> GAMAVLDPEVAQLLSQANEAFVRNDLQVAERLFNEVIKKDARNFAAYETLGDIYQLQGRLNDCCNSWFLAAHLNASDWEFWKIVAILSADLDHVRQAIYCFSRVISLNPMEWESIYRRSMLYKKTGQLARALDGFQRLYMYNPYDANILRELAILYVDYDRIEDSIELYMKVFNANVERREAILAALENALDSSDEESAAEGEDADEKEPLEQDEDRQMFPDINWKKIDAKYKCIPFDWSSLNILAELFLKLAVSEVDGIKTIKKCARWIQRRESQTFW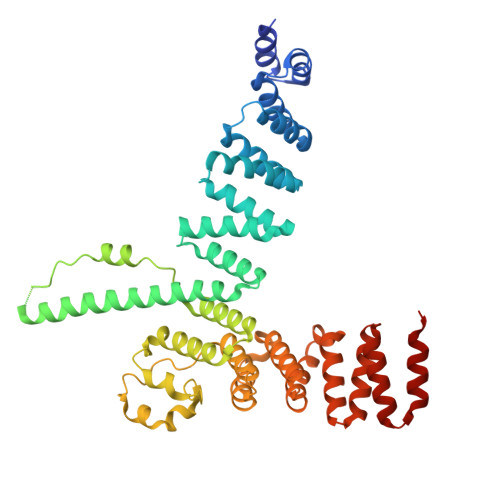DHVPDDSEFDNRRFKNSTFDSLLAAEKEKSYNIPIDIRVRLGLLRLNTDNLVEALNHFQCLYDETFSDVADLYFEAATALTRAEKYKEAIDFFTPLLSLEEWRTTDVFKPLARCYKEIESYETAKEFYELAIKSEPDDLDIRVSLAEVYYRLNDPETFKHMLVDVVEMR> MATGSEASKAAEAVVDWHKHDSKRMLHAVYRVGDLDRTIKYYTECFGMKLLRKRDVPDEKYTNAFLGFGPENTNFAVELTYNYGVDKYDIGTGFGHFAIANDDVYKLAENIKSKGGKITREPGPVKGGSTVIAFAQDPDGYMFELIQRADTPEPLCQVMLRVGDLERSIKFYEKALGMKLLRKKDVPDYKYTIAMLGYADEDKTTVLELTYNYGVTEYSKGNAYAQVAIGTNDVYKSAEAVD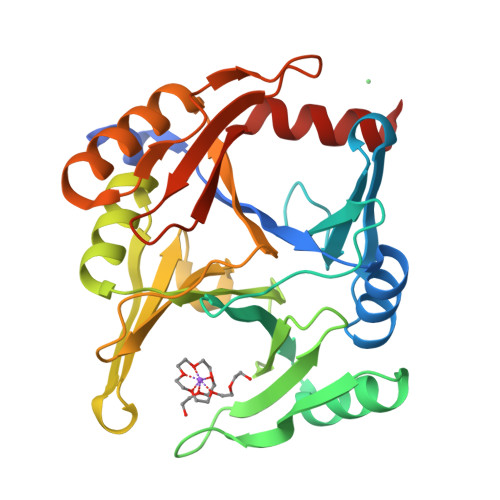LATKELGGKILRQPGPLPGINTKIASFVDPDGWKVVLVDNTDFLKELHLEHHHHHH To reveal the molecular mechanism underpinning the coreceptor role of HS, we solved cryo-electron microscopy structures of three distinct 1:2:1:1 FGF23–FGFR–αKlotho–HS quaternary complexes featuring the ‘c’ splice isoforms of FGFR1 (FGFR1c), FGFR3 (FGFR3c) or FGFR4 as the receptor component. Contrary to our prediction, all three cryo-EM structures reveal identical asymmetric 1:2:1:1 FGF23–FGFR–αKlotho–HS quaternary assemblies in which HS enables a 1:1:1 FGF23–FGFR–αKlotho ternary complex to recruit a lone FGFR chain (termed FGFRS to differentiate it from the ‘primary’ receptor FGFRP within the ternary complex). At the membrane distal end of each quaternary complex, HS engages in tripartite interactions with juxtaposed HS binding sites of FGF23, FGFRP and FGFRS. In doing so, HS augments interactions of FGF23 and FGFRP from the FGF23–FGFRP–αKlotho ternary complex with the FGFRS chain, and thus induces receptor (that is, FGFRP–FGFRS) dimerization.

The direct FGFRP–FGFRS contacts bury a modest solvent-exposed surface area (1542.6 Å2) and are preserved among the three cryo-EM structures. Akin to the FGFRP–FGFRS interface, the FGF23–FGFRS interface is also conserved among the three quaternary complexes and masks a rather modest surface exposed area (1668.6 Å2). Notably, in all three cryo-EM structures, electron densities for the FGF23 N terminus are poorly defined, which implies that the FGF23 N terminus engages FGFRS D3 in a rather degenerate and flexible fashion. We targeted site 2 of the FGFRP–FGFRS interface in each of the three quaternary complexes by introducing four different point mutations individually into full-length FGFR1c (E249A, R254A, I256A, Y280A), FGFR3c (E247A, R252A, I254A, Y278A) or FGFR4 (E243A, R248A, I250A, Y274A). As in the case of the L6-FGFR1cWT cell line, cotreatment with FGF23 and soluble αKlotho of L6-FGFR3cWT and L6-FGFR4WT cell lines robustly stimulated FGFR signalling as detected by phosphorylation/activation of FGFRs and downstream PLCγ1/FRS2α/ERK signal transducers. In contrast, cells expressing mutated FGFR1c, FGFR3c and FGFR4 had diminished FGFR A-loop tyrosine phosphorylation and reduced PLCγ1, FRS2α and MAPK activation. It is unlikely that the impaired signalling by FGFR1cI256A and FGFR4I250A is solely due to reduced cell-surface expression because the glycosylation and cell-surface expression of the corresponding FGFR3cI254A is unaffected.

> EPGDGAQTWARFSRPPAPEAAGLFQGTFPDGFLWAVGSAAYQTEGGWQQHGKGASIWDTFTHHPLAPPGDSRNASLPLGAPSPLQPATGDVASDSYNNVFRDTEALRELGVTHYRFSISWARVLPNGSAGVPNREGLRYYRRLLERLRELGVQPVVTLYHWDLPQRLQDAYGGWANRALADHFRDYAELCFRHFGGQVKYWITIDNPYVVAWHGYATGRLAPGIRGSPRLGYLVAHNLLLAHAKVWHLYNTSFRPTQGGQVSIALSSHWINPRRMTDHSIKECQKSLDFVLGWFAKPVFIDGDYPESMKNNLSSILPDFTESEKKFIKGTADFFALCFGPTLSFQLLDPHMKFRQLESPNLRQLLSWIDLEFNHPQIFIVENGWFVSGTTKRDDAKYMYYLKKFIMETLKAIKLDGVDVIGYTAWSLMDGFEWHRGYSIRRGLFYVDFLSQDKMLLPKSSALFYQKLIEKNGFPPLPENQPLEGTFPCDFAWGVVDNYIQVDTTLSQFTDLNVYLWDVHHSKRLIKVDGVVTKKRKSYCVDFAAIQPQIALLQEMHVTHFRFSLDWALILPLGNQSQVNHTILQYYRCMASELVRVNITPVVALWQPMAPNQGLPRLLARQGAWENPYTALAFAEYARLCFQELGHHVKLWITMNEPYTRNMTYSAGHNLLKAHALAWHVYNEKFRHAQNGKISIALQADWIEPACPFSQKDKEVAERVLEFDIGWLAEPIFGSGDYPWVMRDWLNQRNNFLLPYFTEDEKKLIQGTFDFLALSHYTTILVDSEKEDPIKYNDYLEVQEMTDITWLNSPSQVAVVPWGLRKVLNWLKFKYGDLPMYIISNGIDDGLHAEDDQLRVYYMQNYINEALKAHILDGINLCGYFAYSFNDRTAPRFGLYRYAADQFEPKASMKHYRKIIDSNGFPGPETLERFCPEEFTVCTECSF;> YPNASPLLGSSWGGLIHLYTATARNSYHLQIHKNGHVDGAPHQTIYSALMIRSEDAGFVVITGVMSRRYLCMDFRGNIFGSHYFDPENCRFQHQTLENGYDVYHSPQYHFLVSLGRAKRAFLPGMNPPPYSQFLSRRNEIPLIHFNTPIPRQHTQSAEDDSERDPLNVLKPRARMTPAP;>[2x]TGAPYWTRPERMDKKLLAVPAANTVRFRCPAAGNPTPSISWLKNGREFRGEHRIGGIKLRHQQWSLVMESVVPSDRGNYTCVVENKFGSIRQTYTLDVLERSPHRPILQAGLPANQTAVLGSDVEFHCKVYSDAQPHIQWLKHVEVNGSKVGPDGTPYVTVLKTAGANTTDKELEVLSLHNVTFEDAGEYTCLAGNSIGFSHHSAWLVVLP>[2x]GSHMILKREHFDEKQAQLYDVIIAGGGAGGLSAAVYLARYNLKVLVIEKGRGRSFWMQDLWNYVPRVVSGKELIEGGKEMALHYGADWLNGFVEAVTDTGEEFQVRVKYRFKNSDYPVFRAKYLIAATGLMDVLPQLENMQNVYEYAGYNLHVCLICDGYEMT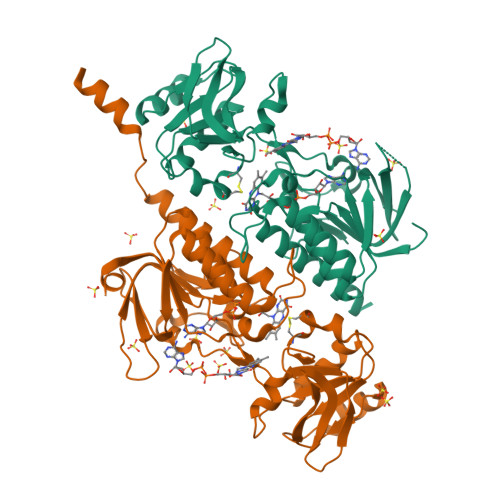NRRAALIAGSEKAINTAFVLNWFTPYITVLTLGAYPVGDEMRAKLADHGYPLIEKPIARFLGKDHVMDGIEFADGTSIKVDTGLISMGSIRHDGYLKNLDLLTDGGDIVTEYDCRTSHPRVFALGDLKKGLNQVSIAVADGTLAATAIWKEIRRASAPRKWTAPLQEAAARAEESARPEISLGAPRGG>MESRVTPVAVIGMGCRLPGGINSPDKLWESLLRGDDLVTEIPPDRWDADDYYDPEPGVPGRSVSRWGGFLDDVAGFDAEFFGISEREATSIDPQQRLLLETSWEAIEHAGLDPASLAGSSTAVFTGLTHEDYLVLTTTAGGLASPYVVTGLNNSVASGRIAHTLGLHGPAMTFDTACSSGLMAVHLACRSLHDGEADLALAGGCAVLLEPHASVAASAQGMLSSTGRCHSFDADADGFVRSEGCAMVLLKRLPDALRDGNRIFAVVRGTATNQDGRTETLTMPSEDAQVAVYRAALAAAGVQPETVGVVEAHGTGTPIGDPIEYRSLARVY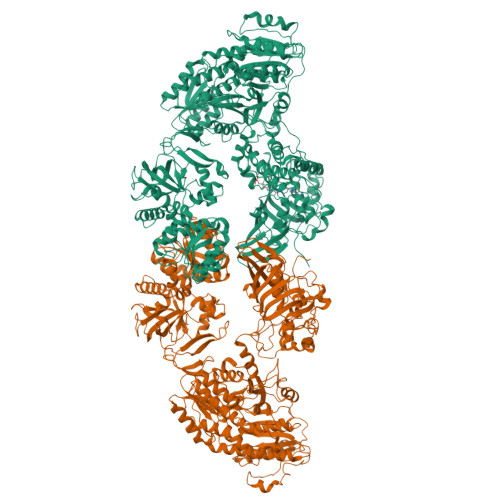GAGTPCALGSAKSNMGHSTASAGTVGLIKAILSLRHGVVPPLLHFNRLPDELSDVETGLFVPQAVTPWPNGNDHTPKRVAVSSFGMSGTNVHAIVEEAPAEASAPESSPGDAEVGPRLFMLSSTSSDALRQTARQLATWVEEHQDCVAASDLAYTLARGRAHRPVRTAVVAANLPELVEGLREVADGDALYDAAVGHGDRGPVWVFSGQGSQWAAMGTQLLASEPVFAATIAKLEPVIAAESGFSVTEAITAQQTVTGIDKVQPAVFAVQVALAATMEQTYGVRPGAVVGHSMGESAAAVVAGALSLEDAARVICRRSKLMTRIAGAGAMGSVELPAKQVNSELMARGIDDVVVSVVASPQSTVIGGTSDTVRDLIARWEQRDVMAREVAVDVASHSPQVDPILDDLAAALADIAPMTPKVPYYSATLFDPREQPVCDGAYWVDNLRNTVQFAAAVQAAMEDGYRVFAELSPHPLLTHAVEQTGRSLDMSVAALAGMRREQPLPHGLRGLLTELHRAGAALDYSALYPAGRLVDAPLPAWTHARLFIDDDGQEQRAQGACTITVHPLLGSHVRLTEEPERHVWQGDVGTSVLSWLSDHQVHNVAALPGAAYCEMALAAAAEVFGEAAEVRDITFEQMLLLDEQTPIDAVASIDAPGVVNFTVETNRDGETTRHATAALRAAEDDCPPPGYDITALLQAHPHAVNGTAMRESFAERGVTLGAAFGGLTTAHTAEAGAATVLAEVALPASIRFQQGAYRIHPALLDACFQSVGAGVQAGTATGGLLLPLGVRSLRAYGPTRNARYCYTRLTKAFNDGTRGGEADLDVLDEHGTVLLAVRGLRMGTGTSERDERDRLVSERLLTLGWQQRALPEVGDGEAGSWLLIDTSNAVDTPDMLASTLTDALKSHGPQGTECASLSWSVQDTPPNDQAGLEKLGSQLRGRDGVVIVYGPRVGDPDEHSLLAGREQVRHLVRITRELAEFEGELPRLFVVTRQAQIVKPHDSGERANLEQAGLRGLLRVISSEHPMLRTTLIDVDEHTDVERVAQQLLSGSEEDETAWRNGDWYVARLTPSPLGHEERRTAVLDPDHDGMRVQVRRPGDLQTLEFVASDRVPPGPGQIEVAVSMSSINFADVLIAFGRFPIIDDREPQLGMDFVGVVTAVGEGVTGHQVGDRVGGFSEGGCWRTFLTCDANLAVTLPPGLTDEQAITAATAHATAWYGLNDLAQIKAGDKVLIHSATGGVGQAAISIARAKGAEIFATAGNPAKRAMLRDMGVEHVYDSRSVEFAEQIRRDTDGYGVDIVLNSLTGAAQRAGLELLAFGGRFVEIGKADVYGNTRLGLFPFRRGLTFYYLDLALMSVTQPDRVRELLATVFKLTADGVLTAPQCTHYPLAEAADAIRAMSNAEHTGKLVLDVPRSGRRSVAVTPEQAPLYRRDGSYIITGGLGGLGLFFASKLAAAGCGRIVLTARSQPNPKARQTIEGLRAAGADIVVECGNIAEPDTADRLVSAATATGLPLRGVLHSAAVVEDATLTNITDELIDRDWSPKVFGSWNLHRATLGQPLDWFCLFSSGAALLGSPGQGAYAAANSWVDVFAHWRRAQGLPVSAIAWGAWGEVGRATFLAEGGEIMITPEEGAYAFETLVRHDRAYSGYIPILGAPWLADLVRRSPWGEMFASTGQRSRGPSKFRMELLSLPQDEWAGRLRRLLVEQASVILRRTIDADRSFIEYGLDSLGMLEMRTHVETETGIRLTPKVIATNNTARALAQYLADTLAEEQAAAPAASKLAAALEHHHHHH[2x]>SMAHLTMPYVMPGDGEVVGVGEPVAIRFDENIADRGAAEKAIKITTNPPVEGAFYWLNNREVRWRPEHFWKPGTAVDVAVNTYGVDLGEGMFGEDNVQTHFTIGDEVIATADDNTKILTVRVNGEVVKSMPTSMGKDSTPTANGIYIVGSRYKHIIMDSSTYGVPVNSPNGYRTDVDWATQISYSGVFVHSAPWSVGAQGHTNTSHGCLNVSPSNAQWFYDHVKRGDIVEVVNTVGGTLPGIDGLGDWNIPWDQWRAGNAKA[2x]

The transpeptidase LtdMt2 catalyzes the formation of the (3–3) cross-links characteristic of the peptidoglycan layer in the Mycobacterium tuberculosis cell wall. The structure analysis reveals that LdtMt2 folds into three domains: two domains in the N-terminal part, both of which show an immunoglobulin-related fold, and a C-­terminal transpeptidase domain. Combining the structures of the two fragments provides a view of the complete three-domain extramembrane part of LdtMt2 and shows that the protein extends at least 80–100 Å from the plasma membrane into the peptidoglycan layer and thus defines the maximal distance at which cross-links are formed by this enzyme. LdtMt2 (Rv2518c) has been reported to be expressed at the highest level and has been found to be essential for virulence.

The structure of the BC module, which was determined to 1.86 Å resolution using Se-SAD phasing, consists of the B domain with an immunoglobulin-related fold and the catalytic domain belonging to the ErfK/YbiS/YbnG fold family. The crystal asymmetric unit contains two molecules with a monomer–monomer interface of approximately 800 Å2, suggesting crystal-packing contacts rather than dimer formation. The structures of the two molecules in the asymmetric unit in the crystals of the BC module are essentially identical, displaying a Cα r.m.s.d. of 0.3 Å for 259 aligned residues. Two of the acetate ions are located in the active-site cleft of domain C. Finally, each polypeptide chain contains a bound metal ion. The Na+ ion is located at the C-­terminus of a surface helix and is coordinated by the carbonyl O atoms of residues 342 and 345 and by three water molecules. The core of the transpeptidase domain consists of a β-­sandwich formed by two β-sheets packed together. The key residues of the catalytic site, Cys354 and His336, correspond to Cys442 and His421 in the E. faecium homologue. In LdtMt2 the active site is located under a lid formed by a pair of antiparallel β-strands and their connecting loop (residues 298–324) that protrude from the core of the catalytic domain. The large hydrophobic residues of the lid (Tyr298, Tyr308 and Tyr318) and the residues surrounding the entrance to the active site (Tyr330, Phe334 and Trp340) contribute to the closure and to the exclusion of solvent, which may support efficient catalysis. The three tryptophan residues (Trp394, Trp398 and Trp401) in this segment form extensive stacking interactions at the domain interface and are likely to stabilize the relative orientation of the two domains.> GSEDLIDGIIFAANYLGSTQLLSERNPSKNIRMMQAQEAVSRVKRMQKAAKIKKKANSE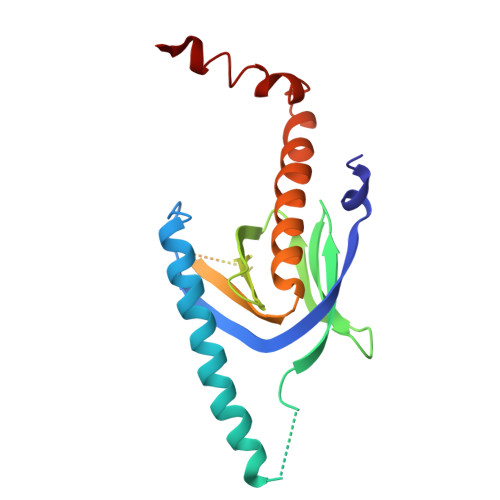GDAQTLTEVDLFISTQRIKVLNADTQETMMDHALRTISYIADIGNIVVLMARRRMPRSASQDCIETTPGAQEGKKQYKMICHVFESEDAQLIAQSIGQAFSVAYQEFLRANGINPEDLSQKEYSDIINTQE>[4x]MGSSHHHHHHMFRTILVANRGEIALRVMRACRELGLRCVAVYSEADRDAPHVAYADDAFLIGPPSPAESYLNIDAIIRAAKATGAEAIHPGYGFLAENASFVRAVTAAGLIFIGPPAEAMERMGGKTAARREATAAGVPVVPGVLEPVTDAAEVRRLGKEFGYPIAIKAVGGGGGRGLRVVRSPEEVDEAFAAARREAEVAFKNGELYVEKYLDDPRHIEIQVLADRYGNAVALGERDCSVQRRHQKLIEECPSPALTPELRAEMGAAAVRLAKAVGYVSAGTLEFLFQDGRYYFLEMNTRIQVEHTVTEMVYGIDLVAAQIRIAQGEKLWFKQEDVVPRGHAIECRINAEDPLHNFRPALGTIGEYHEPVGFGVRVDSGVRAYYTVPSHYDSLLAKLITWGSDRQEA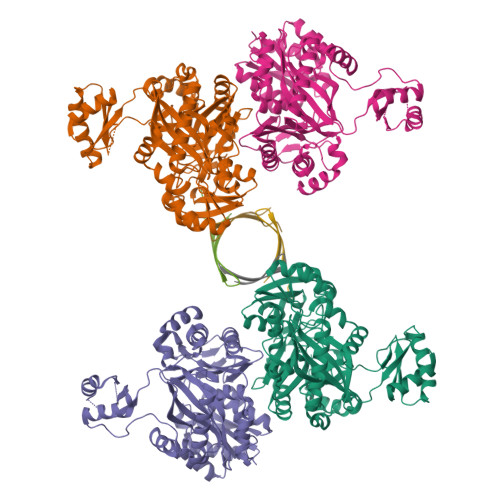IARMRRALAEYRIEGVTTIIPFHQAALEHPVFTAGAATVNFIPRHPELFSRAAELTPPTAA;>SAGAEPAPEPRRFTIEVNGRRFGVAVFGDGMNATPVASPSRSAPARRAAPKKTTLAAPVDAVISPIQGRVVAVRVAHGQQVEAGQVLFIVEAMKMENEITAPHSGTIAEVRVEVGTTVEAGAMLATYQNTANNTNGK[4x]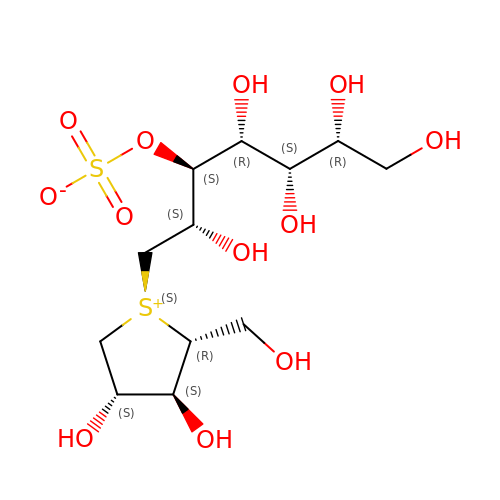(1S,2R,3S,4R)-1-{(1S)-2-[(2R,3S,4S)-3,4-dihydroxy-2-(hydroxymethyl)tetrahydrothiophenium-1-yl]-1-hydroxyethyl}-2,3,4,5-tetrahydroxypentyl sulfate | C12 H24 O12 S2 | OMKXVFDVAGCPBS-WJKNVNJGSA-N> MNKTYAACPQNWIGVENKCFYFSEYPSNWTFAQAFCMAQEAQLARFDNQDELNFLMRYKANFDSWIGLHRESSEHPWKWTD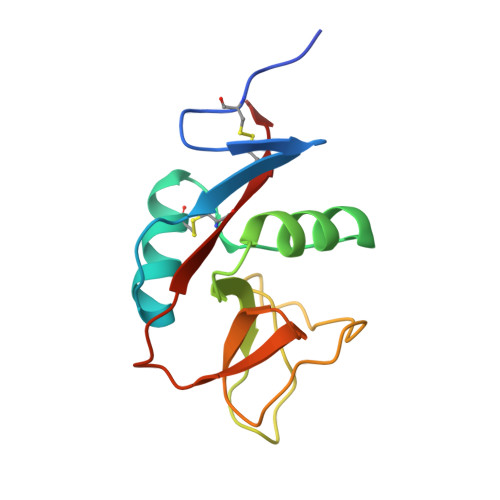NTEYNNTIPIRGEERFAYLNNNGISSTRIYSLRMWICSKLNAS> MSSFLPEGGCYELLTVIGKGFEDLMTVNLARYKPTGEYVTVRRINLEACSNEMVTFLQGELHVSKLFNHPNIVPYRATFIADNELWVVTSFMAYGSAKDLICTHFMDGMNELAIAYILQGVLKALDYIHHMGYVHRSVKASHILISVDGKVYLSGLRSNLSMISHGQRQRVVHDFPKYSVKVLPWLSPEVLQQNLQGYDAKSDIYSVGITACELANGHVPFKDMPATQMLLEKLNGTVPCLLDTSTIPAEELTMSPSRSVANSGLSDSLTTSTPRPSNGDSPSHPYHRTFSPHFHHFVEQCLQRNPDARPSASTLLNHSFFKQIKRRASEALPELL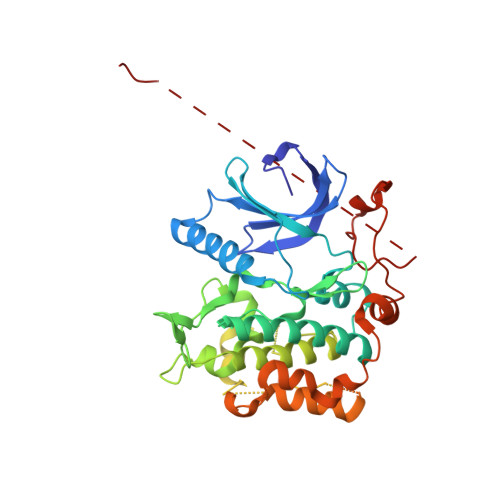RPVTPITNFEGSQSQDHSGIFGLVTNLEELEVDDWEF>ARKCSLTGKWTNDLGSNMTIGAVNSRGEFTGTYTTAVTATSNEIKESPLHGTQNTINKRTQPTFGFTVNWKFSESTTVFTGQCFIDRNGKEVLKTMWLLRSSVNDIGDDWKATRVGINIFTRLRT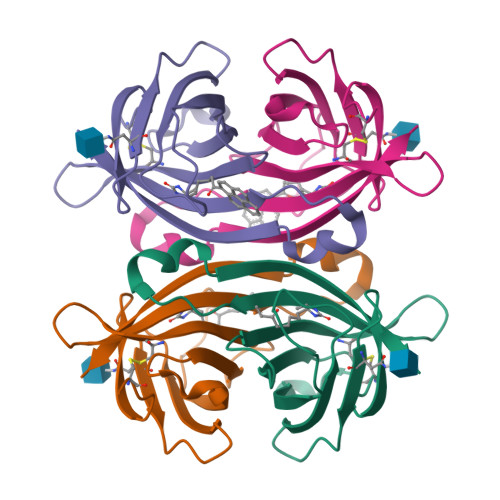QKE[4x]>[2x]MGSSHHHHHHSSGRENLYFQGMIYMPIVVAVDKKSDRAERVLRFAAEEARLRGVPVYVVHSLPGGGRTKDEDIIEAKETL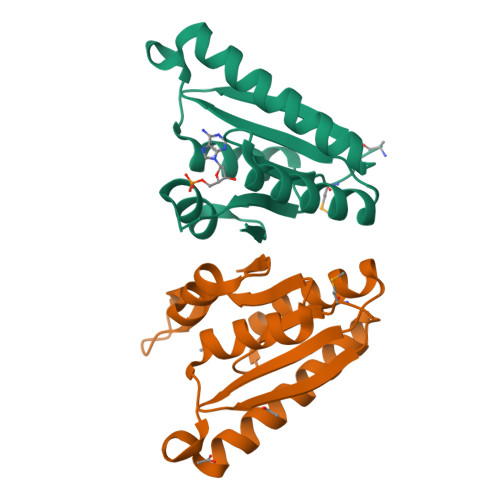SWAVSIIRKEGAEGEEHLLVRGKEPPDDIVDFADEVDAIAIVIGIRKRSPTGKLIFGSVARDVILKANKPVICIK>[3x]SITTPEQGTTVGGVIAEPSVQMSAAADMATGKSVDSEWEAFFSFHTSVNWSTSETQGKILFKQSLGPLLNPYLTHLAKLYVAWSGSIEVRFSISGSGVFGGKLAAIVVPPGIEPIQSTSMLQYPHVLFDARQVEPVIFTIPDLRSTLYHLMSDTDTTSLVIMIYNDLINPYANDSNSSGCIVTVETKPGPDFKFHLLKPPGSMLTHGSVPCDLIPKSSSLWIGNRFWSDITDFVIRPFVFQANRHFDFNQETAGWSTPRFRPITV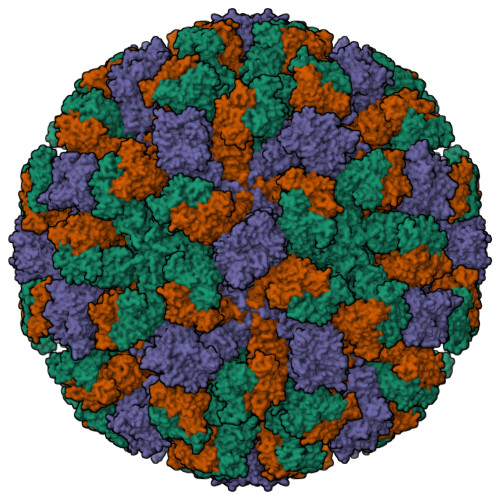TISQKEGEMLGIGVATDYIVPGIPDGWPDTTIPNELIPAGDYAITNQSGNDIQTKEEYESAMIISNNTNFKSMYICGSLQRAWGNKKVSNTAFITTATVKENKLIPSNTIDQTKIAIFQDNHVNRDVQTSDDTLALLGYTGIGEEAIGADREKVVRIGVLPEAGARGGNHPIFYRNSMKLGYVIKSIDVFNSQILHTSRQLSLNNYLLSPDSFAVYRIIDSNGSWFDIGIDSDGFSFVGVSSIGKLEFPLTASYMGNQLAKIRLASNIR> VSLARRPLPPL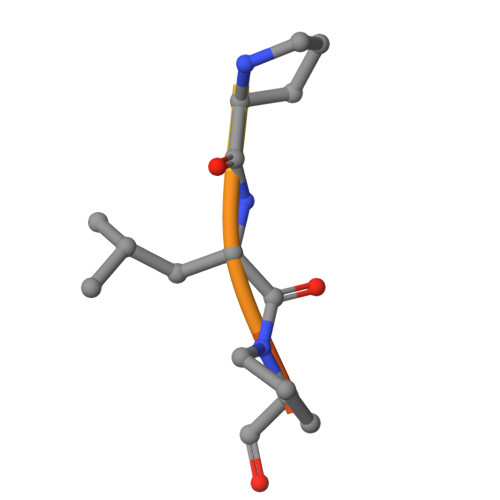P>[4x]SYADTFTEFTNVEEAKKWGNAQYKKYGLSKPEQEAIKFYTRDASKINGPLRANQGNENGLPADILQKVKLIDQSFSKMKMPQNIILFRGDDPAYLGPEFQDKILNKDGTINK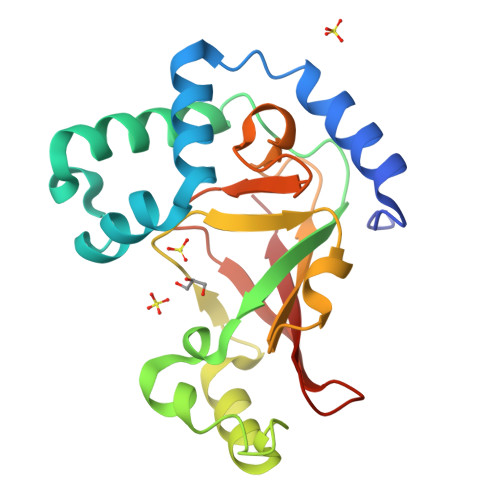TVFEQVKAKFLKKDRTEYGYISTSLMSAQFGGRPIVTKFKVTNGSKGGYIDPISYFPGQLEVLLPRNNSYYISDMQISPNNRQIMITAMIFK> TAPTPILRFVAVGDWGGVPNAPFHTAREMANAKAIATTVKTLGADFILSLGDNFYFTGVHDAKDKRFQETFEDVFSDPSLRNVPWHVLAGNHDHLGNVSAQIAYSKISKRWNFPSPYYRLRFKIPRSNVSVAIFMLDTVTLCGNSDDFVSQQPERPRNLALARTQLAWIKKQLAAAKEDYVLVAGHYPVWSIAEHGPTHCLVKQLLPLLTTHKVTAYLCGHDHNLQYLQDENGLGFVLSGAGNFMDPSKKHLRKVPNGYLRFHFGAENSLGGFAYVEITPKEMSVTYIEASGKSLFKTK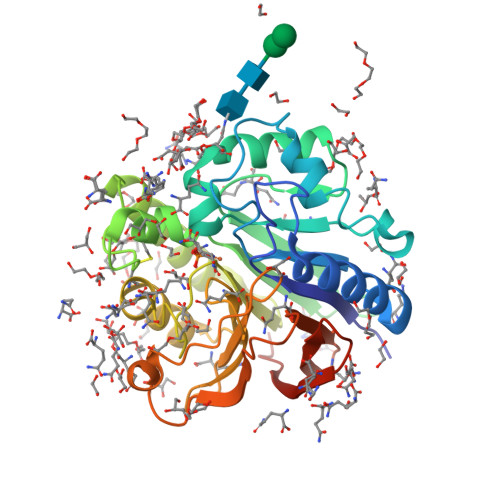LPRRARSEHQHRRA ICV, however, has only one major surface glycoprotein, the hemagglutinin-esterase-fusion (HEF) protein, which possesses all-in-one of receptor binding, receptor destroying and membrane fusion activities. To further evaluate the infectivity and transmissibility of IDV, we expressed and purified the ectodomain of D/OK HEF, and determined that it also uses 9-O-Acetyl-Sia as its receptor by glycan microarray. We also solved the crystal structure of D/OK HEF, both in its native state (resolution of 2.4 Å) and in complex with its receptor analogue (resolution of 3.1 Å), and the structure of the enzymatically inactive HEF (resolution of 2.4 Å) alone and in complex with two receptor analogs respectively (both resolutions of 2.2 Å). Indeed, our results show that IDV HEF is functionally and structurally similar to ICV HEF, but with some distinct characteristics.

In our IDV HEF complex structure with its receptor analogue 9-N-Ac-Sia, we found that the 9-N-acetyl group of the substrate was tilted up against the oxyanion hole as the covalent modification of S57 by arsenic blocked the insertion of the 9-N-acetyl group inserting into enzymatic site. Due to the presence of cacodylate buffer in the crystallization conditions, S57 in our IDV HEF structure is covalently modified by the addition of a dimethylarsenic group. The covalent modification of active site serine by arsenic was first reported by Ian Wilson’s group in 2003, when they solved the structure of an acetyl esterase, HerE, and its complex with the inhibitor dimethylarsinic acid, and illustrated the mechanism of the broad scope inhibition of serine hydrolases by As(V)-containing organic compounds. The active-site architecture of the HEF sialate-9-O-acetylesterase is fully conserved in ICV and IDV HEF with S57, D356 and H359 creating a catalytic triad and with the side chain of N117 and the NH groups of S57 and G85 forming an oxyanion hole. The esterase pocket of IDV HEF is highly conserved among ICV and nidovirus HE proteins and could represent a potential drug target for developing broad-spectrum inhibitors.

> ELICIVQRVNESFSLHSGFGGNVYSMKTEPMTGFTNVTKGASVINQKDWIGFGDSRTDLTNDQFPASSDVPLAVAKKFRSLSGASLMLSAFGPPGKVDYLYQGCGKEKVFYEGVNWSPEAGIDCFGSNWTQTKKDFYSRIYEAARSSTCMTLVNSLDTKISSTTATAGTASSCSSSWMKSPLWYAESSVNPGAKPQVCGTEQSATFTLPTSFGIYKCNKHVVQLCYFVYENKAKFNTFGCGDYYQNYYDGNGNLIGGMDNRVAAYRGIANAGVKIECPSKILNPGTYSIKSTPRFLLVPKRSYCFDTDGGYPIQVVQSEWSASRRSDNATEEACLQTEGCIFIKKTTPYVGEADDNHGDIEMRQLLSGLGNNDTVCVSQSGYTKGETPFVKDYLSPPKYGRCQLKTDSGRIPTLPSGLIIPQAGTDS;> IFGIDDLIFGLLFVGFVAGGVAGGYFWGRSNGGGGGASVSSTQAGFDKIGKDIQQLRNDTNAAIEGFNGRIAHDEQAIKNLAKEIEDARAEALVGELGIIRSLIVANISMNLKESLYELANQITKRGGGIAQEAGPGCWYVDSENCDASCKEYIFNFNGSATVPTL> M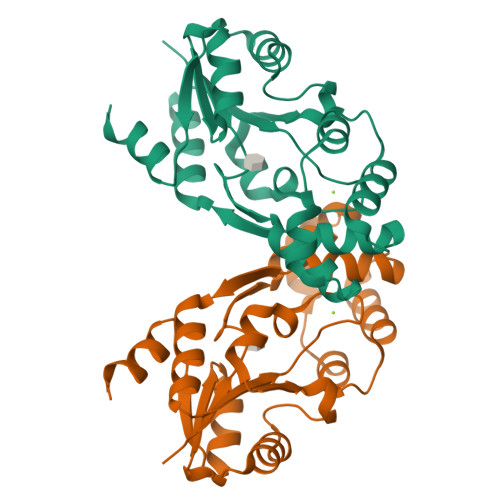ARKEAKMLYIFDLGNVIVDIDFNRVLGAWSDLTRIPLASLKKSFHMGEAFHQHERGEISDEAFAEALCHEMALPLSYEQFSHGWQAVFVALRPEVIAIMHKLREQGHRVVVLSNTNRLHTTFWPEEYPEIRDAADHIYLSQDLGMRKPEARIYQHVLQAEGFSPSDTVFFDDNADNIEGANQLGITSILVKDKTTIPDYFAKVLC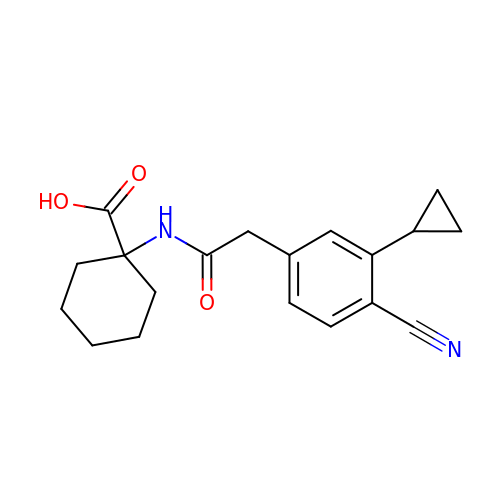1-{[(4-cyano-3-cyclopropylphenyl)acetyl]amino}cyclohexane-1-carboxylic acid | C19 H22 N2 O3 | XZXSSWDGVSHUNZ-UHFFFAOYSA-N>[2x]MTGPILSGLDPRFERTLYAHVGKEGSWTLDYYLRHGGYETAKRVLKEKTPDEVIEEVKRSGLRGRGGAGFPTGLKWSFMPKDDGKQHYLICNADESEPGSFKDRYILEDVPHLLIEGMILAGYAIRATVGYIYVRGEYRRAADRLEQAIKEARARGYLGKNLFGTDFSFDLHVHRGAGAYICGEETALMNSLEGLRANPRLKPPFPAQSGLWGKPTTINNVETLASVVPIMERGADWFAQMGTEQSKGMKLYQISGPVKRPGVYELPMGTTFRELIYEWAGGPLEPIQAIIPGGSSTPPLPFTEEVLDTPMSYEHLQAKGSMLGTGGVILIPERVSMVDAMWNLTRFYAHESCGKCTPCREGVAGFMVNLFAKIGTGQGEEKDVENLEALLPLIEGRSFCPLADAAVW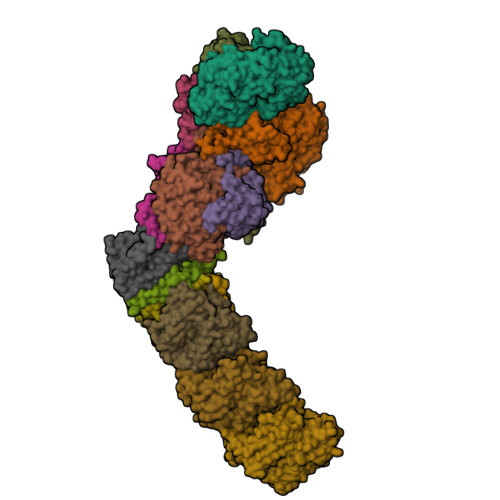PVKGSLRHFKDQYLALAREKRPVPRPSLWR;>[2x]MGFFDDKQDFLEETFAKYPPEGRRAAIMPLLRRVQQEEGWIRPERIEEIARLVGTTPTEVMGVASFYSYYQFVPTGKYHLQVCATLSCKLAGAEELWDYLTETLGIGPGEVTPDGLFSVQKVECLGSCHTAPVIQVNDEPYVECVTRARLEALLAGLRAGKRLEEIELPGKCGHHVHEVEV;>[2x]MVRVKVNDRIVEVPPGTSVMDAVFHAGYDVPLFCSEKHLSPIGACRMCLVRIGLPKKGPDGKPLLNEKGEPEIQWQPKLAASCVTAVADGMVVDTLSDVVREAQAGMVEFTLLNHPLDCPTCDKGGACELQDRTVEYGLYEKYYQKGPLELPVYTRFEFTRRHVDKHHPLSPFVILDRERCIHCKRCVRYFEEVPGDEVLDFIERGVHTFIGTMDFGLPSGFSGNITDICPVGALLDLTARFRARNWEMEETPTTCALCPVGCGITADTRSGELLRIRAREVPEVNEIWICDAGRFGHEWADQNRLKTPLVRKEGRLVEATWEEAFLALKEGLKEARGEEVGLYLAHDATLEEGLLASELAKALKTPHLDFQGRTAAPASLFPPASLEDLLQADFALVLGDPTEEAPILHLRLSEFVRDLKPPHRYNHGTPFADLQIKERMPRRTDKMALFAPYRAPLMKWAAIHEVHRPGEEREILLALLGDKEGSEMVAKAKEAWEKAKNPVLILGAGVLQDTVAAERARLLAERKGAKVLAMTPAANARGLEAMGVLPGAKGASWDEPGALYAYYGFVPPEEALKGKRFVVMHLSHLHPLAERYAHVVLPAPTFYEKRGHLVNLEGRVLPLSPAPIENGEAEGALQVLALLAEALGVRPPFRLHLEAQKALKARKVPEAMGRLSFRLKELRPKERKGAFYLRPTMWKAHQAVGKAQEAARAELWAHPETARAEALPEGAQVAVETPFGRVEARVVHREDVPKGHLYLSALGPAAGLRVEGRVLVPAGGEA;>[2x]MREEFLEEIPLDAPPEEAKELRTEVMTLNVGPQHPSTHGVLRLMVTLSGEEVLEVVPHIGYLHTGFEKTMEHRTYLQNITYTPRMDYLHSFAHDLAYALAVEKLLGAVVPPRAETIRVILNELSRLASHLVFLGTGLLDLGALTPFFYAFRERETILDLFEWVTGQRFHHNYIRIGGVKEDLPEEFVPELKKLLEVLPHRIDEYEALFAESPIFYERARGVGVIPPEVAIDLGLTGGSLRASGVNYDVRKAYPYSGYETYTFDVPLGERGDVFDRMLVRIREMRESVKIIKQALERLEPGPVRDPNPQITPPPRHLLETSMEAVIYHFKHYTEGFHPPKGEVYVPTESARGELGYYIVSDGGSMPYRVKVRAPSFVNLQSLPYACKGEQVPDMVAIIASLDPVMGDVDR;>MRLERVLEEARAKGYPIEDNGLGNLWVVLPRERFKEEMAHYKAMGFNFLADIVGLDYLTYPDPRPERFAVVYELVSLPGWKDGDGSRFFVRVYVPEEDPRLPTVTDLWGSANFLEREVYDLFGIVFEGHPDLRKILTPEDLEGHPLRKDYPLGETPTLFREGRYIIPAEFRAALTGKDPGLTFYKGGSRKGYRSLWADLKKAREVKG[2x];>MALKDLFERDVQELEREGILFTTLEKLVAWGRSNSLWPATFGLACCAIEMMASTDARNDLARFGSEVFRASPRQADVMIVAGRLSKKMAPVMRRVWEQMPDPKWVISMGACASSGGMFNNYAIVQNVDSVVPVDVYVPGCPPRPEALIYAVMQLQKKVRGQAYNERGERLPPVAAWKRTRG[2x];>[2x]MSASSERELYEAWVELLSWMREYAQAKGVRFEKEADFPDFIYRMERPYDLPTTIMTASLSDGLGEPFLLADVSPRHAKLKRIGLRLPRAHIHLHAHYEPGKGLVTGKIPLTKERFFALADRAREALAFA;>MTLKALAQSLGITLKYLFSKPVTVPYPDAPVALKPRFHGRHVLTRHPNGLEKCIGCSLCAAACPAYAIYVEPAENDPENPVSAGERYAKVYEINMLRCIFCGLCEEACPTGAIVLGYDFEMADYEYSDLVYGKEDMLVDVVGTKPQRREAKRTGKPVKVGYVVPYVRPELEGFKAPTEGGKR[2x];>[2x]MAPIQEYVGTLIYVGVALFIGVAALLVGALLGPKKPGRAKLMPYESGNDPAGEVKRFPVHFYVVAMLFILFDVEVAFLWPYAVSAGGLGLYGFLGVLAFTLLLFVGFLYEWWKGVMRWH;>[2x]MTWSYPVDPYWMVALKALLVVVGLLTAFAFMTLIERRLLARFQVRMGPNRVGPFGLLQPLADAIKSIFKEDIVVAQADRFLFVLAPLISVVFALLAFGLIPFGPPGSFFGYQPWVINLDLGILYLFAVSELAVYGIFLSGWASGSKYSLLGSLRSSASLISYELGLGLALLAPVLLVGSLNLNDIVNWQKEHGWLFLYAFPAFLVYLIASMAEAARTPFDLPEAEQELVGGYHTEYSSIKWALFQMAEYIHFITASALIPTLFLGGWTMPVLEVPYLWMFLKIAFFLFFFIWIRATWFRLRYDQLLRFGWGFLFPLALLWFLVTALVVALDLPRTYLLYLSALSFLVLLGAVLYTPKPARKGGGA;>[2x]MSLLEGLALFLLLLSGVLVVTLRNAIHAALALILNFLVLAGVYVALDARFLGFIQVIVYAGAIVVLFLFVIMLLFAAQGEIGFDPLVRSRPLAALLALGVAGILAAGLWGLDLAFTQDLKGGLPQALGPLLYGDWLFVLLAVGFLLMAATVVAVALVEPGKASRAKEAEKREEVAR;>[2x]MSYLLTSALLFALGVYGVLTRRTAILVFLSIELMLNAANLSLVGFARAYGLDGQVAALMVIAVAAAEVAVGLGLIVAIFRHRESTAVDDLSELRG;>[2x]MALLGTILLPLLGFALLGLFGKRMREPLPGVLASGLVLASFLLGAGLLLSGGARFQAEWLPGIPFSLLLDNLSGFMLLIVTGVGFLIHVYAIGYMGGDPGYSRFFAYFNLFIAMMLTLVLADSYPVMFIGWEGVGLASFLLIGFWYKNPQYADSARKAFIVNRIGDLGFMLGMAILWALYGTLSISELKEAMEGPLKNPDLLALAGLLLFLGAVGKSAQIPLMVWLPDAMAGPTPVSALIHAATMVTAGVYLIARSSFLYSVLPDVSYAIAVVGLLTAAYGALSAFGQTDIKKIVAYSTISQLGYMFLAAGVGAYWVALFHVFTHAFFKALLFLASGSVIHALGGEQDVRKMGGLWKHLPQTRWHALIGALALGGLPLLSGFWSKDAILAATLTYPFGGVGFYVGALLVAVLTAMYAMRWFVLVFLGEERGHHHPHEAPPVMLWPNHLLALGSVLAGYLALPHPLPNVLEPFLKPALAEVEAHHLSLGAEWGLIALSAAVALLGLWAGFVFFQRKVFPAWYLAFEAASREAFYVDRAYNALIVNPLKALAEALFYGDRGLLSGYFGLGGAARSLGQGLARLQTGYLRVYALLFVLGALLLLGVMRW;>[2x]MVVLAVLLPVVFGALLLLGLPRALGVLGAGLSFLLNLYLFLTHPGGVAHAFQAPLLPGAGVYWAFGLDGLSALFFLTIALTVFLGALVARVEGRFLGLALLMEGLLLGLFAARDLLVFYVFFEAALIPALLMLYLYGGEGRTRALYTFVLFTLVGSLPMLAAVLGARLLSGSPTFLLEDLLAHPLQEEAAFWVFLGFALAFAIKTPLFPLHAWLPPFHQENHPSGLADALGTLYKVGVFAFFRFAIPLAPEGFAQAQGLLLFLAALSALYGAWVAFAAKDFKTLLAYAGLSHMGVAALGVFSGTPEGAMGGLYLLAASGVYTGGLFLLAGRLYERTGTLEIGRYRGLAQSAPGLAALALILFLAMVGLPGLSGFPGEFLTLLGAYKASPWLAALAFLSVIASAAYALTAFQKTFWEEGGSGVKDLAGAEWGFALLSVLALLLMGVFPGYFARGLHPLAEAFAKLLGGGA;>MTLAILAVFSVALTLLGFVLPPQGVKRATLLGLALALASLLLTWGKPFAFGPYAVDGVSQVFTLLALLGALWTVGLVRSGRFEFYLLVLYAALGMHLLASTRHLLLMLVALEALSLPLYALATWRRGQGLEAALKYFLLGALAAAFFLYGAALFYGATGSLVLGAPGEGPLYALALGLLLVGLGFKAALAPFHFWTPDVYQGSPTPVVLFMATSVKAAAFAALLRVAAPPEALALLVALSVVVGNLAALAQKEAKRLLAYSSIAHAGYMALALYTGNAQALGFYLLTYVLATGLAFAVLSQISPDRVPLEALRGLYRKDPLLGLAFLVAMLSLLGLPPLAGFWGKYLAFAEAARAGAWGVLVLALVTSAVSAYYYLGLGLAVFARPEETPFRPGPPWARAAVVAAGVLLLALGLLPGLVLPALAAGG[2x];>[2x]MVRVGMRAAPRVSLEALKAALGGLKLSEAKVYLITDWQDKRDQARYALLLHTGKKDLLVPDAFGPAFPGGEEALSELVGLLLAQGARRFYEAVVSPGEMTALLDLPPEELLKRVMAIANPTDPGIYLKRAA> MPEITRRRALTAAAAVAATASAAVTLAAPAASAAGHHEPAAPESFDEVYKGRRIQGRPARGAAHHHEHGGGYEVFVDGVQLHVMRNADGSWISVVSHYDPVPTPRAAARAAVDELQGAPLLPFP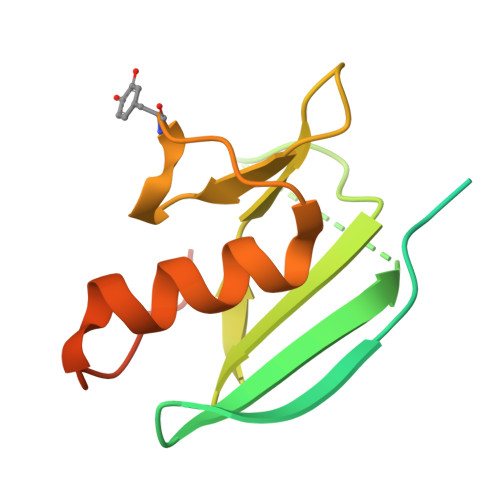ANLEHHHHHH> MGIRNRLSELLSERGLKISRVAKDVKIARSSLTSMAQNDSEMIRYDAIDKLCSYLHISPSEFFEHNPINFDFTFDEEPNYKINDVFEGFEVTANITHAFSIENFDFEILVDVELDNRQKLNFDLDVSY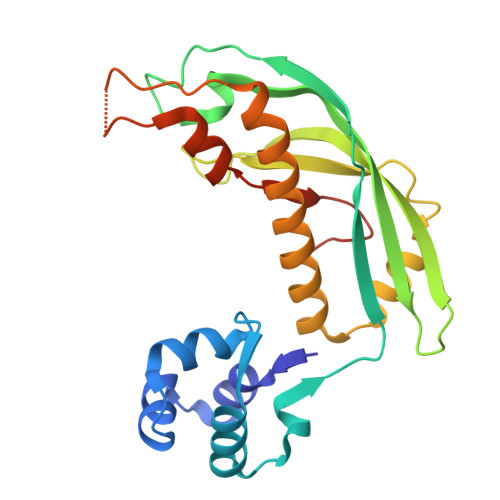KETEKITNSQHRFIFTIKNEDENIGLKKYVDSLSAGLKNLLFKKINQKLSGYVSEIIVKNIDDIEELFPNKGEKSTTLHKEILQTDSRLSSDIFKEYGSHHHHHH>[2x]TLKNSDAYVIRPFMPSDEETLYDLCLKSCIENS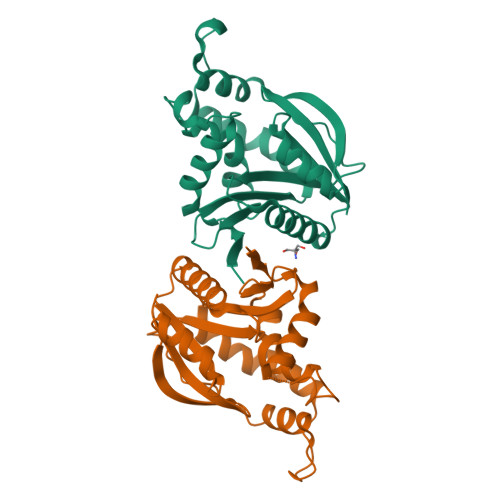NGDEIYKREPRIIGDRDLGAYIYLHPEYIYVLEDDRDKICGYLCGALDSKQFYERYESEWLTQIRDRHPQPENDIASWTPEEIVANSFYNFTPPTDVSVLYLSHLEARFDSSVPEKVIKRIIRFILEQLKAKGSYGASMLIDSWRTNLRRIFTSMGFVDLQEYSWMSEQKCMIAIKLM>MAHHHHHHVGTMIPLIYHPIYSQLDLPVGHRYPINKYRLLYEEIVRQREQSEAWQASFEFHTPIAAELSRITPLHDPDYVQALLEGRLPAAKMRRIGFPWSKTLIERTLHSVGGTCLTVEQALQSGVAIHLSGGYHHAHADFGSGFCLFNDLAIAAHFALSLPSVDKVLIIDSDVHHGDGTATLCAERDDIITLSFHCDKNFPARKPASSMDVGFANQTGDEEFLSTFIQVVEMAVNLHRPDLILYDAGVDIHNDDELGYLSISQAAIAQRDRFMLGLAKQESIPIACVIGGGYREDHAALVPLHLELLKAALLSAGY[2x]

Classical Zn2+-dependent deac(et)ylases play fundamental regulatory roles in life and are well characterized in eukaryotes regarding their structures, substrates and physiological roles. Structurally, these enzymes are composed of a central eight-stranded parallel β-sheet flanked by α-helices on each site, known as the α/β-arginase/deacetylase fold. All active site residues were conserved, as shown by the multiple sequence alignment and the structural alignment, suggesting a general acid/base catalytic mechanism for the bacterial enzymes as described for the eukaryotic counterparts. These enzymes mediate catalysis using a penta-coordinated catalytic Zn2+ ion coordinated by two aspartates and a histidine (KpHdaH (1b): Asp181, Asp269, His183).

We solved the X-ray crystal structures of KpHdaH (1b), RwDmhA (1b), and VcHdaH (5b) in complexes with SAHA to a resolution of 1.95 Å, 1.75 Å, and 1.64 Å, respectively. As described for mammalian Zn2+-dependent HDACs, the hydroxamates coordinated the catalytic Zn2+-ion in a bidentate fashion, the carbonyl oxygen replacing the carbonyl oxygen of the acetamide in the substrate and the hydroxyl group replacing the position of the catalytic water molecule. For all structures, we confirmed the binding of the inhibitors within the substrate binding tunnel with the catalytically important Y of the XGGY-motif forming a hydrogen bond to the carbonyl oxygen of the hydroxamate group. For cluster 5, the enzyme of Vibrio cholerae HdaH of sub-cluster 5b, VcHdaH (5b), was a monomer in solution, as confirmed by the crystal structure and by analytical size-exclusion chromatography. We identified VcHdaH (5b) being an active de-decanoylase. We were not able to perform inhibitor studies with VcHdaH (5b) because the observed de-decanoylase activity was neither strong enough to perform Michaelis–Menten kinetics nor to determine Ki/IC50 values. Whether VcHdaH (5b) is inhibited by the HDAC11-selective trapoxin A analog TD034173 or recently reported HsHDAC11-selective hydroxamates needs further investigation.Hydrogen sulfide (H2S) plays roles in many physiological processes in mammals, including relaxation of vascular smooth muscles, regulation of inflammation, and inhibition of insulin signaling. More recently, it has been proposed that sulfane sulfurs, i.e., sulfur atoms with oxidation state 0 or −1, existing in the form of polysulfides (H2Sn), glutathione persulfide (GSSH), glutathione trisulfide (GSSSG), cysteine persulfide (CysSSH) and so on, actually mediate some of the reported biological activities previously thought to be regulated by H2S67891011. We determined the crystal structures of the m3MST complexes with 1 and 3 at high resolution. The most remarkable feature is that C248 is persulfurated in both crystal structures.

Persulfurated C248 appears to interact with the 4-pyrimidone-like aromatic ring of both compounds. To our knowledge, this interaction is novel in terms of both the long distance (>3.45 Å) and the orientation of the persulfide bond (almost perpendicular to the aromatic ring of the inhibitors). Direct hydrogen bonding by R188 and S250 and water-mediated hydrogen bonding by E195 and R197 are commonly observed with compounds 1 and 3. In addition, compound 1 forms water-mediated hydrogen bonds with D63 and H74. Both compounds were in van der Waals contact with W36, L38, P39, D73, H74, Y108, R188, P196, R197, G249, S250, V252 and V277. The thiophene ring (compound 1) and naphthalene ring (compound 3) exhibit cation-π interaction with R197 and parallel stacking interaction with the salt bridge between D73 and R19726. Gas-phase calculations indicated that the interaction of S–S− with pyrimidone is strongly exothermic (10.4 kcal/mol; CCSD(T)/aug-cc-pVDZ), which is not inconsistent with the experimental ITC measurements (ΔH = −9.37 and −11.76 kcal/mol for compounds 1 and 3, respectively). We concluded that the interaction is predominantly due to electrostatic attraction between the persulfur anion and the positively charged carbonyl carbon of the pyrimidone structure. Compound 1 showed about 25% inhibition of recombinant CBS and CSE enzymatic activities, while compound 3 was almost inactive towards CBS and CSE. The side chain of R197 of h3MST is positioned inside the active site and forms a hydrogen bond with pyruvate, whereas that of m3MST-inhibitor complexes is directed outside of the active site and forms a hydrogen bond with D73. The arginine residues in the substrate binding site have been reported to be critical residues in determining substrate specificity for 3MST41, and this difference may be due to the binding molecule, i.e., compound 3 and pyruvate.

>[2x]QLFRALVSAQWVAEALKAPRSSQPLKLLDASWYLPKLGRDARREFEERHIPGAAFFDIDRSSDHTSPYDHMLPNATHFADYAGSLGVSAATHVVIYDGSDQGLYSAPRVWWMFRAFGHHSVSLLDGGFRHWLNQNLPISSGKSHSEPAEFSAQLDPSFIKTHEDILENLDARRFQVVDARAAGRFQGTQPEPRDGIEPGHIPGSVNIPFTEFLTNEGLEKSPEEIKRLFKEKKVDLSKPLVATCGSGVTASHVVLGAFLSGKSDVPVYDGSWVEWYMRAQPEHIISEGRGKTQ>[8x]GMRKHPQTATKHLFVSGGVASSLGKGLTASSLGQLLTARGLHVTMQKLDPYLNVDPGTMNPFQHGEVFVTEDGAETDLDVGHYERFLDRNLPGSANVTTGQVYSTVIAKERRGEYLGDTVQVIPHITDEIKRRILAMAQPDADGNRPDVVITEIGGTVGDIESQPFLEAARQVRHYLGREDVFFLHVSLVPYLAPSGELKTKPTQHSVAALRSIGITPDALILRCDRDVPEALKNKIALMCDVDIDGVISTPDAPSIYDIPKVLHREELDAFVVRRLNLPFRDVDWTEWDDLLRRVHEPHETVRIALVGKYVELSDAYLSVAEALRAGGFKHRAKVEICWVASDGCETTSGAAAALGDVHGVLIPGGFGIRGIEGKIGAIAYARARGLPVLGLCLGLQCIVIEAARSVGLTNANSAEFDPDTPDPVIATMPD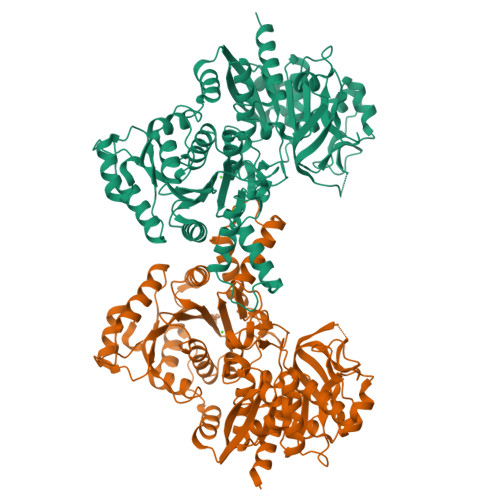QEEIVAGEADLGGTMRLGSYPAVLEPDSVVAQAYQTTQVSERHRHRYEVNNAYRDKIAESGLRFSGTSPDGHLVEFVEYPPDRHPFVVGTQAHPELKSRPTRPHPLFVAFVGAAIDYKAGELLPVEIPEIPEHTPNGSSHRDGVGQPLPEPASRG>PLHSIISSTESVQGSTSKHEFQAETKKLLDIVARSLYSEKEVFIRELISNASDALEKLRHKLVSDGQALPEMEIHLQTNAEKGTITIQDTGIGMTQEELVSNLGTIARSGSKAFLDALQNQAEASSKIIGQFGVGFYSAFMVADRVEVYSRSAAPGSLGYQWLSDGSGVFEIAEASGVRTGTKIIIHLKSDCKEFSSEARVRDVVTKYSNFVSFPLYLNGRRMNTLQAIWMMDPKDVREWQHEEFYRYVAQAHDKPRYTLHYKTDAPLNIRSIFYVPDMKPSMFDVSRELGSSVALYSRKVLIQTKATDILPKWLRFIRGVVDSEDIPLNLSRELLQESALIRKLRDVLQQRLIKFFIDQSKKDAEKYAKFFEDYGLFMREGIVTATEQEVKE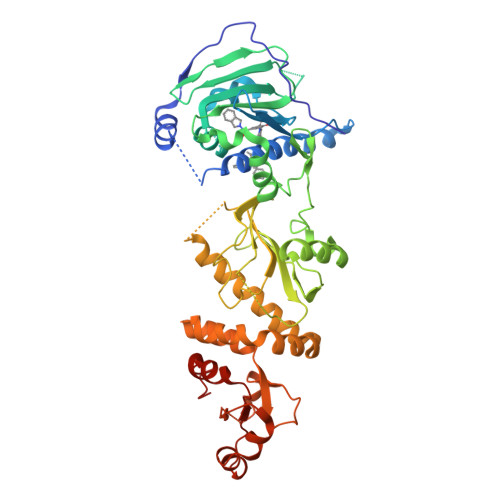DIAKLLRYESSALPSGQLTSLSEYASRMRAGTRNIYYLCAPNRHLAEHSPYYEAMKKKDTEVLFCFEQFDELTLLHLREFDKKKLISVET[2x]> KVFERCELARTLKRLGMDGYRGISL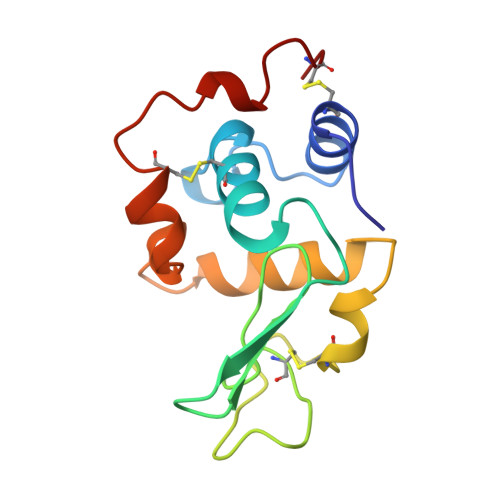ANWMCLAKWESGYNTRATNYNAGDRSTDYGIFQINSRYWCNDGKTPGAANAAHLSCSALLQDNIADAVAAAKRVVRDPQGIRAWVAWRNRCQNRDVRQYVQGCGV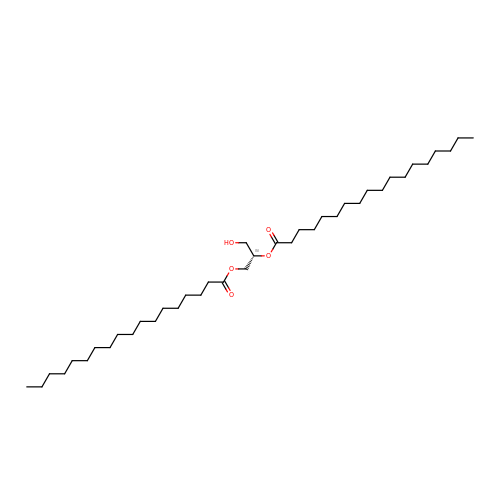DIACYL GLYCEROL | C39 H76 O5 | UHUSDOQQWJGJQS-QNGWXLTQSA-N4-(hydroxymethyl)-1-[[2-(3-methoxyphenyl)-1,3-thiazol-5-yl]methyl]piperidin-4-ol 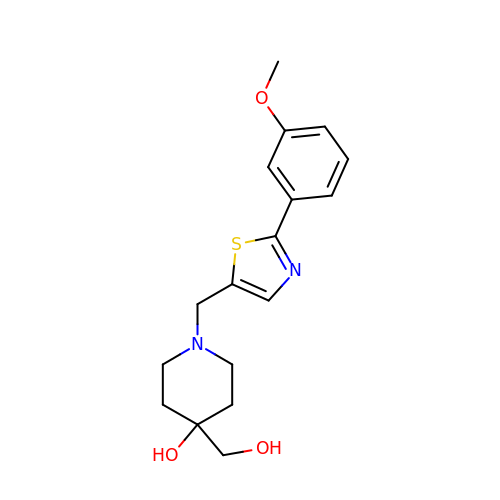| C17 H22 N2 O3 S | FXCZNKJONOHACS-UHFFFAOYSA-N>GPKK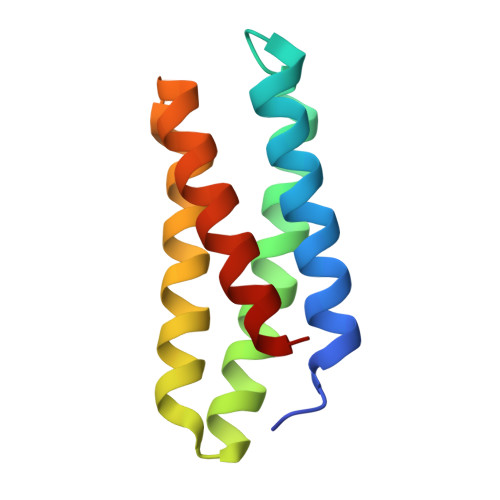KIQIMAEEALKDALSILNIVKTNSPPAEEQLERFAKRFERNLWGIARLFESGDQKDEAEKAKRMIEWMKRIKTTASEDEQEEMANAIITILQSWFFS[8x]To validate the versatility of the VIALS workflow, we used two different IMPs, archaerhodopsin-3 (AR3) and the human adenosine A2A receptor (hA2AR), as proof of concept. AR3, from the archaebacterium Halorubrum sodomense, is a light-driven proton pump that undergoes a sequence of conformational changes induced by the absorption of a photon and is commonly used in optogenetic experiments. hA2AR is a class A G-protein-coupled receptor that is expressed in the cardiovascular, respiratory, immune and central nervous systems, and is implicated in immunosuppression and the regulation of sleep. However, the production of integral membrane protein microcrystals in lipidic cubic phase at the desired crystal density and quantity is challenging. This paper introduces VIALS (versatile approach to high-density microcrystals in lipidic cubic phase for serial crystallography), a simple, fast and efficient method for preparing hundreds of microlitres of high-density microcrystals suitable for serial X-ray diffraction experiments at both synchrotron and free-electron laser sources. Using the VIALS approach, room-temperature structures are reported of (i) the archaerhodopsin-3 protein in its dark-adapted state and 110 ns photocycle intermediate, determined to 2.2 and 1.7 Å, respectively, and (ii) the human A2A adenosine receptor in complex with two different ligands determined to a resolution of 3.5 Å.

Here we report two room-temperature AR3 structures: the first, by SSX, is the dark-adapted state of the protein; the second, by time-resolved SFX, is the 110 ns photocycle intermediate. AR3 microcrystals in LCP (5–10 µm) were taken to SACLA and time-resolved SFX data were collected as described in Section 2.4. The LCP thread with a high density of microcrystals was continuously ejected from the high-viscosity sample injector and a femtosecond pump–probe experiment was performed with a time delay of 110 ns. With a crystal hit rate of up to 31% (determined by the SACLA real-time data-processing pipeline; Nakane et al., 2016), a full data set was obtained within 2.5 h using only ∼60 µl of crystal-laden LCP. A total of 11 912 frames were successfully indexed in the space group P212121 and the high quality of the diffraction data was supported by the figures of merit R split and CC1/2 of 16.1 and 99.2%, respectively. The AR3110 ns final structure was refined to 1.7 Å resolution with an R work and R free of 18.12 and 19.64%, respectively. The resulting electron-density maps revealed the presence of 61 water molecules and lipid fragments. The mean B-factor value of 36.0 Å2 is also within the values reported for a room-temperature structure of 1.7 Å.

> QAGYDLLGDGRPETLWLGIGTLLMLIGTFYFLVRGWGVTDKDAREYYAVTILVPGIASAAYLSMFFGIGLTEVTVGGEMLDIYYARYADWLFTTPLLLLDLALLAKVDRVTIGTLVGVDALMIVTGLIGALSHTAIARYSWWLFSTICMIVVLYFLATSLRSAAKERGPEVASTFNTLTALVLVLWTAYPILWIIGTEGAGVVGLGIETLLFMVLDVTAKVGFGFILLRSRAILGDTEAPEPSAGADVSAAD>[3x]MKTFIFLALLGAAVAFPVDDDDKIVGGYTCGANTVPYQVSLNSGYHFCGGSLINSQWVVSAAHCYKSGIQVRLGEDNINVVEGNEQFISASKSIVHPSYNSNTLNNDIMLIKLKSAASLNSRVASISLPTSCASAGTQCLISGWGNTKSSGTS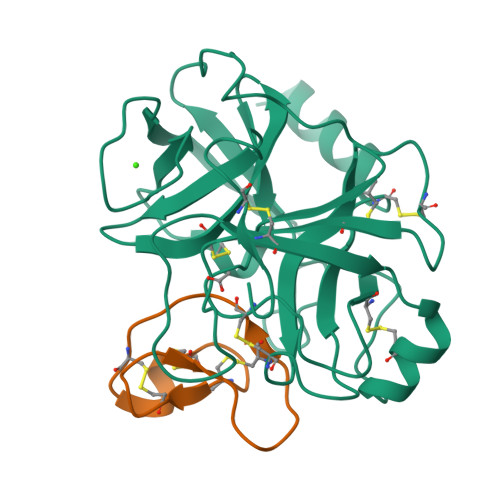YPDVLKCLKAPILSDSSCKSAYPGQITSNMFCAGYLEGGKDSCQGDSGGPVVCSGKLQGIVSWGSGCAQKNKPGVYTKVCNYVSWIKQTIASN;>[3x]SGSDGGVCPKILKKCRRDSDCPGACICRGNGYCG> MPNVSLTAKGGGHYIEDQWDTQVVEAGVFDDWWVHVEAWNKFLDNLRGINFSVASSRSQ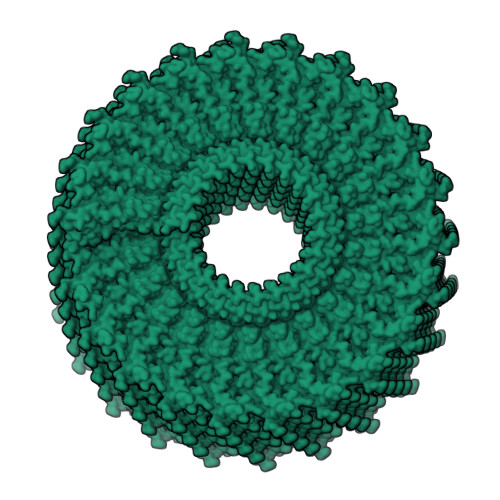VAEYLAALDRDLPADVDRRFAGARGQIGSPNYLPAPKFFRLDKRTIAELTRLSRLTDQPHNNRDIELNRAKRATTNPSPPAQAPSENLTLRDVQPLKDSALHYQYVLIDLQSARLPVYTRKTFERELALEWIIPDAEEA>GMIEELGKIDRIIQESVPGKQITLAHVIAAPIEAVYECLGVDHEGAIGVVSLTPNETAIIAA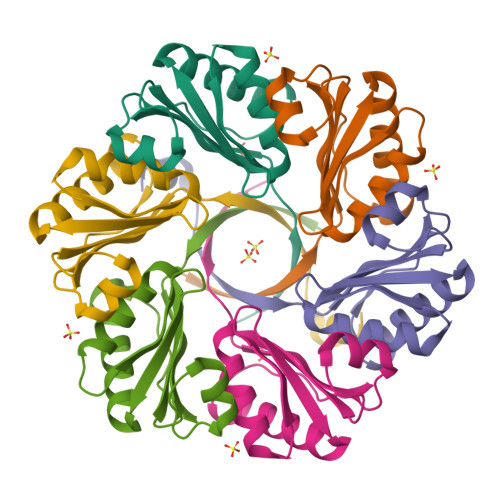DIAGAAANIDICFVDRFTGSVMFSGDIQSVETSLEDILEYFKNSLGFSTVPLTKS[3x]> NLFQFAKMING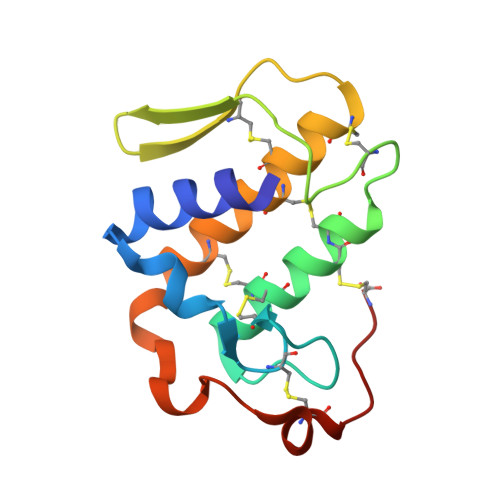KLGAFSVWNYISYGCYCGWGGQGTPKDATDRCCFVHDCCYGRVRGCNPKLAIYSYSFKKGNIVCGKNNGCLRDICECDRVAANCFHQNKNTYNKNYKFLSSSRCRQTSEQC>MSLDRPRCCLRGKECSINRFQQVESRWGYSGTSDRIRFSVNKRI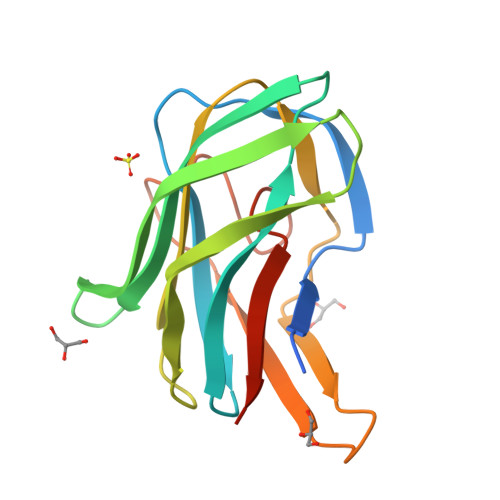FVVGFGLYGSIHGPTDYQVNIQIIHTDSNTVLGQNDTGFSCDGSASTFRVMFKEPVEVLPNVNYTACATLKGPDSHYGTKGMRKVTHESPTTGAKTCFTFCYAAGNNNGTSVEDGQIPEVIFYTEGHHHHHH[2x]> IVGGYTCAANSIPYQVSLNSGSHFCGGSLINSQWVVSAAHCYKSRIQVRLGEHNIDVLEGNEQFINAAKIITHPNFNGNTLDNDIMLIKLSSPATLNSRVATVSLPRSCAAAGTECLISGWGNTKSSGSSYPSLLQCLKAPVLSDSSCKSSYPGQITGNMICVGFLEGGKDSCQGDSGGPVVCNGQLQGIVSWGYGCAQKNKPGVYTKVCNYVNWIQQTIAAN;> VPMDCSRYPNTTSEEGK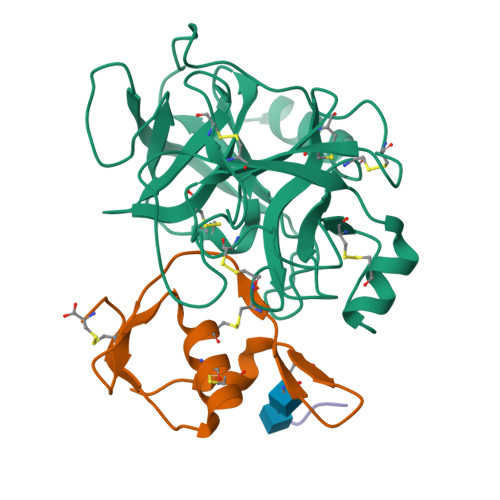VMILCNKALNPVCGTDGVTYDNECVLCAHNLEQGTSVGKKHDGEC;> TNEE LmrR is a transcriptional repressor regulating the expression of the multidrug ABC transporter LmrCD. In the apo state, LmrR shows high affinity for the promotor region of LmrRCD. This affinity is reduced upon binding of a drug at its drug-binding site, enabling expression of the multidrug transporter. LmrR is a homodimeric protein with the drug binding site at the dimer interface.19 Central in this binding site are two Trp residues, W96 and W96′ (residue 96 from the other monomer), oriented face-to-face at 7 Å from each other.

To investigate the importance of π–π interactions for drug binding, the electron density in the π electron cloud of W96 was modulated by progressive fluorination of the W96 indole side chain. To assess whether the Trp analogs influence the overall structure of LmrR and its drug-binding pocket, crystal structures were determined of LmrR with bound Dau for LmrR variants 5FW, 5,6diFW, and 5,6,7triFW. The crystal structures belong to the same crystal form (space group C2 with very similar unit cell dimensions) and were refined to resolutions varying between 2.55 and 2.15 Å. Although the crystal structures show generally good geometry, they all suffer from high crystallographic B-factors (average B-factors for protein atoms varying between ∼57 and ∼89 Å2), indicative of static disorder in the crystals. Nevertheless, the electron density maps were of sufficient quality to identify the Trp analogs at positions 67 and 96 in both polypeptide chains of the dimeric LmrR variants. No major differences were observed in the backbone and side chain conformations around residues W67 and W96, compared to wild-type LmrR.19 Moreover, as shown in Figures 2 and S6, the binding mode of Dau to LmrR is not substantially affected by the presence of the fluorinated Trp analogs. Dau is bound in the same way as in the wild-type protein, with the aromatic part of Dau sandwiched between two Trp analog residues, stabilized by π–π stacking interactions. Thus, we conclude that the different Dau binding affinities observed for the LmrR variants are not related to conformational changes of the protein or significantly altered ligand binding modes. The binding affinities of LmrR for Dau and RBF decreased upon increasing degrees of fluorination of W96. Dau behaved less extreme, with the kd decreasing 6-fold.

>[2x]MAEIPKEMLRAQTNVILLNVLKQGDNYVYGIIKQVKEASNGEMELNEATLYTIFKRLEKDGIISSYXGDESQGGRRKYYRLTEIGHENMRLAFESXSRVDKIIENLEANKKSEAIK4-[(4-{4-[(E)-2-cyanoethenyl]-2,6-dimethylphenoxy}thieno[3,2-d]pyrimidin-2-yl)amino]-2-fluorobenzonitrile 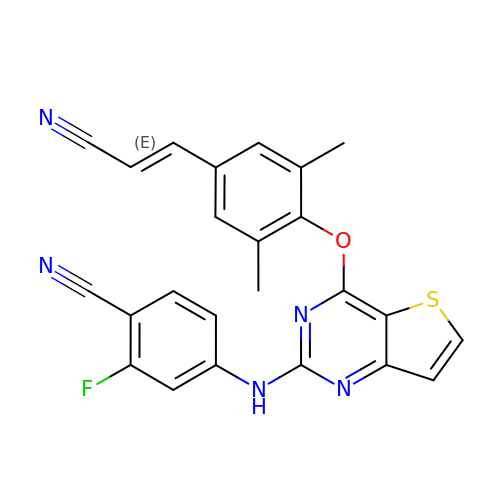| C24 H16 F N5 O S | WJBQILBCHRFMQR-ONEGZZNKSA-N>X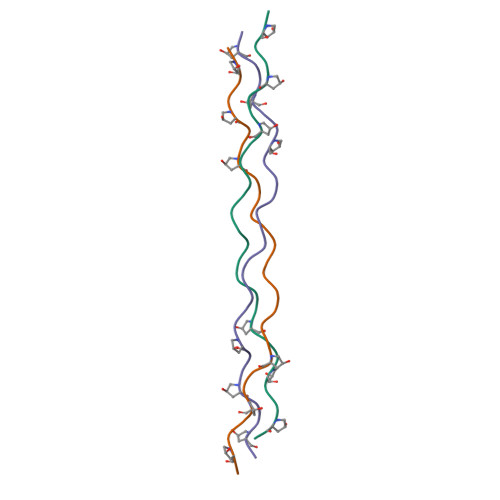PPGPPGPPGDDGPSGAEGPPGPPGPPGX[3x]>GMADPPSLHHEAQPLKFIAVDYCPESCTHSPESSTITLTFDHRGGSRWRSTTRFQYGTFSSLIQCPKGNTSGLNFNIYLSSLEGDKSQDAIDFEFLGKDKRIVQTNYYTAGTGNREAIHDLGFDCSDGFHEYVIKWGPDLIQWLIDGKVIRSVRADGEGFPQKPMFLYASVWDASYIDEGRWTGPYVGCDAPYICLY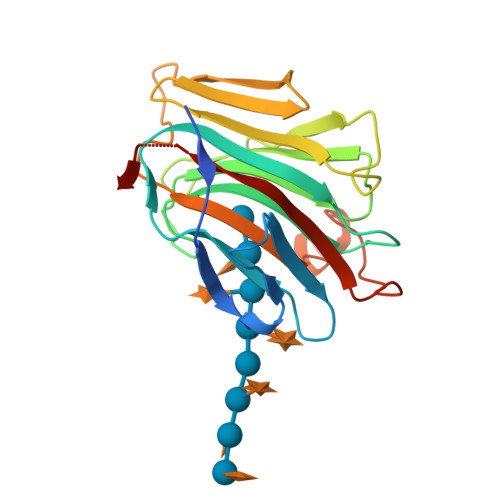KNVNVPVGTAVE[2x]> AEYVRALFDFNGNDEEDLPFKKGDILRIRDKPEEQWWNAEDSE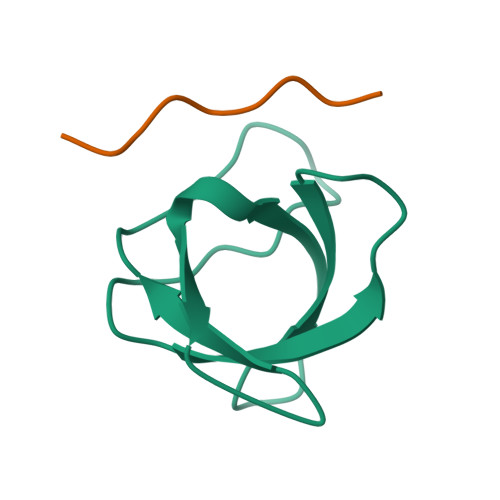GKRGMIPVPYVEKY;> PPPALPPKKR> MARRKCRNRFVKKNGQCNVEFTNMDDKPQRYIADMFTTCVDIRWRYMLLLFSLAFLVSWLLFGLIFWLIALIHGDLENPGGDDTFKPCVLQ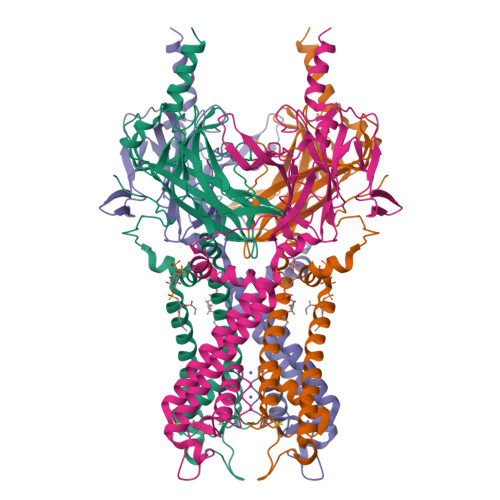VNGFVAAFLFSIETQTTIGYGFRCVTEECPLAVFMVVVQSIVGCIIDSFMIGAIMAKMAAPKKRAQTLLFSHNAVVAMRDGKLCLMWRVGNLRKSHIVEAHVRAQLIKPRITEEGEYIPLDQIDIDVGFDKGLDRIFLVSPITILHEINEDSPLFGISRQDLETDDFEIVVILEGMVEATAMTTQARSSYLASEILWGHRFEPVLFEEKNQYKVDYSHFHKTYEVPSTPRCSAKDLVENKFLLSNSLEVLFQ>GTGPDKLKKVLDKLRLKRKDISEAAETVNKVVERLLRRMQKRESEFKGVEQLNTGSYYEHVKISAPNEFDVMFKLEVPRIELQEYYETGAFYLVKFKRIPRGNPLSHFLEGEVLSATKMLSKFRKIIKEEVKEIKDIDVSVEKEKPGSPAVTLLIRNPEEISVDIILALESKGSWPISTKEGLPIQGWLGTKVRTNLRREPFYLVPKNAKDGNSFQGETWRLSFSHTEKYILNNHGIEKTCCESSGAKCCRKECLKLMKYLLEQLKKEFQELDAFCSYHVKTAIFHMWTQDPQDSQWDPRNLSSCFDKLLAFFLECLRTEKLDHYFIPKFNLFSQELIDRKSKEFLSKKIEYERNNGFPIFDKL[2x]

Cyclic GMP-AMP (cGAMP) synthase (cGAS) is essential for the host defense against cytosolic double-stranded (ds)DNA arising from various maladies (e.g., pathogen invasion, ionizing irradiation, and genotoxic chemicals). Upon directly binding to and dimerizing on dsDNA, cGAS cyclizes ATP and GTP into 2′−5′/3′−5′-linked cGAMP, a unique metazoan second messenger for initiating type-I interferon (IFN-I)-mediated inflammatory responses. cGAS is central to antitumor immunity, host defense against an array of pathogens, and regulating autoimmunity. Here, we resolve these numerous fundamental mechanistic questions in innate immunology and present a unifying catalytic mechanism of cGAS. Finally, we reveal how mouse cGAS achieves more stringent substrate selectivity and higher catalytic efficiency than the human enzyme. Together, we set forth a unifying catalytic mechanism of cGAS in which dsDNA-binding pre-organizes the active site into a rigid yet adaptable lock for two sets of keys (substrates and intermediate) necessary to specifically synthesize 2′−5/3′−5′-cGAMP.

Next, to determine whether Mn2+ is preferred at either metal binding site, we soaked WT-mcGAScat•dsDNA crystals with ATP pre-complexed with increasing concentrations of Mn2+ (0.015-1 mM) in the presence of excess Mg2+ (10 mM); the presence of Mn2+ was tracked via its anomalous signal at 1.8961 Å (6539 eV) during data collection. G The presence of Mn2+ at each indicated concentration for the ATP-bound WT-mcGAScat•dsDNA crystal was monitored by tracking its anomalous signal (contoured at 5σ; the average resolution of maps shown: 2.63 ± 0.11 Å). Here, we found that cGAS specifically favors Mn2+ over Mg2+ by ≥100-fold at the catalytic metal binding site; the binding here also cooperatively increased the affinity for Mn2+ at the first site. Our structures consistently suggest that only one Mg2+ is necessary for productive substrate binding, while the second Mg2+ drives chemistry (i.e., neutralizing negative charges upon deprotonating 2′- or 3′-OH by Asp307). When ATP is bound to mcGAScat•dsDNA at Site-1, its 2′-OH makes H-bonds with Glu371 and Ser368, while the 3′-OH interacts with Lys424 and its own β-phosphate, apparently stabilizing the substrate.N-(1H-indazol-6-yl)acetamide | C9 H9 N3 O 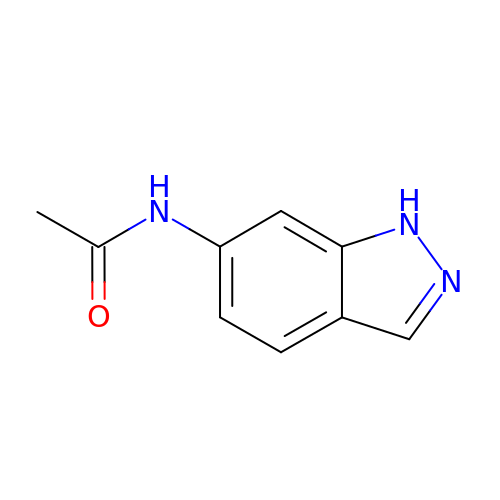| HOQHKYACTYMRFK-UHFFFAOYSA-N>MSWVQLAGHTGSFKAAGTSGLILKRCSEPERYCLARLMADALRGCVPAFHGVVERDGESYLQLQDLLDGFDGPCVLDCKMGVRTYLEEELTKARERPKLRKDMYKKMLAVDPEAPTEEEHAQRAVTKPRYMQWREGISSSTTLGFRIEGIKKADGSCSTDFKTTRSREQVLRVFEEFVQGD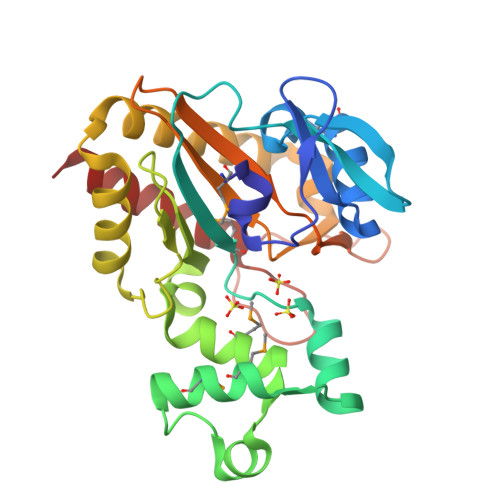EEVLRRYLNRLQQIRDTLEVSEFFRRHEVIGSSLLFVHDHCHRAGVWLIDFGKTTPLPDGQILDHRRPWEEGNREDGYLLGLDNLIGILASLAER[2x]> MGSD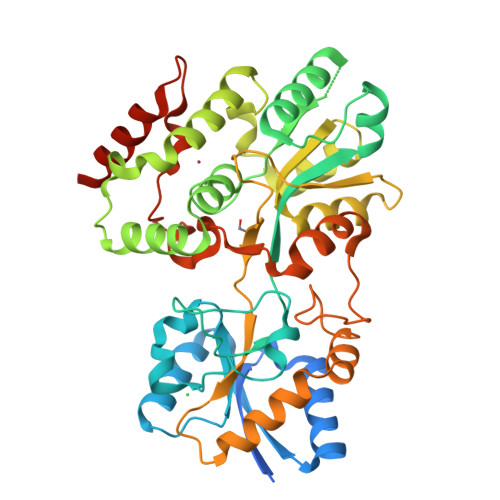KIHHHHHHENLYFQGHGSKEKGKEEEPVRLSVLIREKHYSSGLQNVFTKLELEEGIAVTVETIQDDQYPTVLHARLADGTAPDVVEVSLPSLHALDPYLYFVDLSKEAWIPDLLIPPTDPYGKTFALPLNCAVSINALFYNKDLFDRYGISEPKSWNELLESCALIVKSGISIVPLALSTTESFPHTLLADAITKVLGEQGARDLVKRATDDSIDWTHERALYPVLGAYLELFKRGYVNKHHRTARVREIIHDFTRDRIAMYFGSHLVADAIIKERPGINLGACVLPITENAQDVLTGSLEVQGLAVHKKSARVATACRALSVLASAAYQNSFFEEHKGLPAFRNTTSAVIPACLSALFKSHIEKGKVIQAIDAYAQAQNTPHRASVFPDFAAYVTDPAPTAHTMLHRAQTEARRRREPVQKKE> MPLAFCGTENHSAAYRVDQGVLNNGCFVDALNVVPHVFLLFITFPILFIGWGSQSSKVHIHHSTWLHFPGHNLRWILTFILLFVLVCEIAEGILSDGVTESRHLHLYMPAGMAFMAAITSVVYYHNIETSNFPKLLIALLIYWTLAFITKTIKFVKFYDHAIGFSQLRFCLTGLLVILYGMLLLVEVNVIRVRRYIFFKTPREVKPPEDLQDLGVRFLQPFVNLLSKGTYWWMNAFIKTAHKKPIDLRAIAKLPIAMRALTNYQRLCVAFDAQARKDTQSPQGARAIWRALCHAFGRRLILSSTFRILADLLGFAGPLCIFGIVDHLGKENHVFQPKTQFLGVYFVSSQEFLGNAYVLAVLLFLALLLQRTFLQASYYVAIETGINLRGAIQTKIYNKIMHMSTSNLSMGEMTAGQICNLVAIDTNQLMWFFFLCPNLWTMPVQIIVGVILLYYILGVSALIGAAVIILLAPVQYFVATKLSQAQRTTLEHSNERLKQTNEMLRGMKLLKLYAWESIFCSRVEVTRRKEMTSLRAFAVYTSISIFMNTAIPIAAVLITFVGHVSFFKESDLSPSVAFASLSLFHILVTPLFLLSSVVRSTVKALVSVQKLSEFLSSAEIREEQCAPREPAPQGQAGKYQAVPLKVVNRKRPAREEVRDLLGPLQRLAPSMDGDADNFCVQIIGGFFTWTPDGIPTLSNITIRIPRGQLTMIVGQVGCGKSSLLLATLGEMQKVSGAVFWNSNLPDSEGEDPSSPERETAAGSDIRSRGPVAYASQKPWLLNATVEENITFESPFNKQRYKMVIEACSLQPDIDILPHGDQTQIGERGINLSGGQRQRISVARALYQQTNVVFLDDPFSALDVHLSDHLMQAGILELLRDDKRTVVLVTHKLQYLPHADWIIAMKDGTIQREGTLKDFQRSECQLFEHWKTLMNRQDQELEKETVMERKASEPSQGLPRAMSSRDGLLLDEEEEEEEAAESEEDDNLSSVLHQRAKIPWRACTKYLSSAGILLLSLLVFSQLLKHMVLVAIDYWLAKWTDSALVLSPAARNCSLSQECDLDQSVYAMVFTLLCSLGIVLCLVTSVTVEWTGLKVAKRLHRSLLNRIILAPMRFFETTPLGSILNRFSSDCNTIDQHIPSTLECLSRSTLLCVSALTVISYVTPVFLVALLPLAVVCYFIQKYFRVASRDLQQLDDTTQLPLVSHFAETVEGLTTIRAFRYEARFQQKLLEYTDSNNIASLFLTAANRWLEVCMEYIGACVVLIAAATSISNSLHRELSAGLVGLGLTYALMVSNYLNWMVRNLADMEIQLGAVKRIHALLKTEAESYEGLLAPSLIPKNWPDQGKIQIQNLSVRYDSSLKPVLKHVNTLISPGQKIGICGRTGSGKSSFSLAFFRMVDMFEGRIIIDGIDIAKLPLHTLRSRLSIILQDPVLFSGTIRFNLDPEKKCSDSTLWEALEIAQLKLVVKALPGGLDAIITEGGENFSQGQRQLFCLARAFVRKTSIFIMDEATA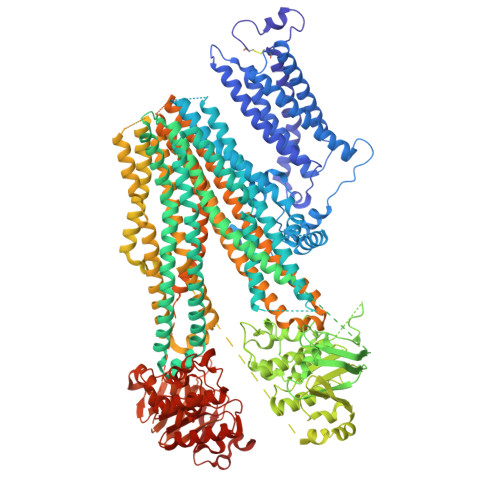SIDMATENILQKVVMTAFADRTVVTIAHRVHTILSADLVMVLKRGAILEFDKPETLLSQKDSVFASFVRADK> GDVEEAIDRAVARVADTMPTGPRNTESVPALTAVETGHTSQVVPGDTMQTRHVKNYHSRTESSIENFLCRAACVYIATYKSAGGTPTERYASWRINTRQMVQLRRKFELFTYLRFDMEITFVITSTQDPGTQLAQDMPVLT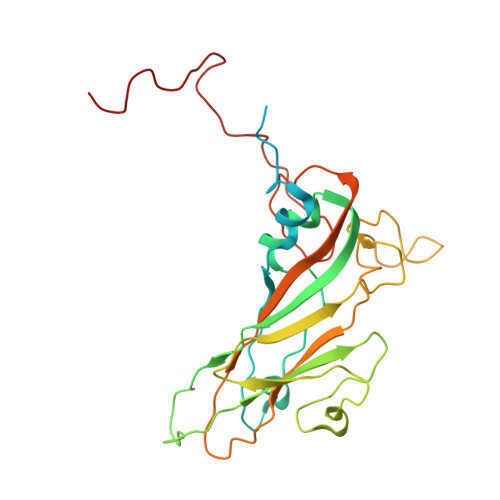HQIMYIPPGGPVPNSATDFAWQSSTNPSIFWTEGCAPARMSVPFISIGNAYSNFYDGWSHFTQEGVYGFNSLNNMGHIYVRHVNEQSLGVSTSTLRVYFKPKHVRAWVPRPPRLSPYVKSSNVNFKPTAVTTERKDINDVGTLRPVGYTNH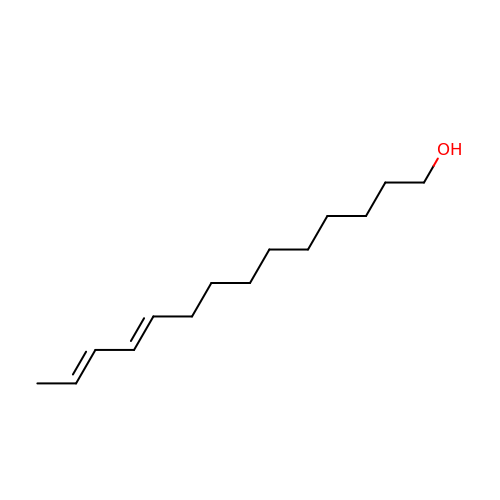(10E,12Z)-tetradeca-10,12-dien-1-ol | C14 H26 O | SDYZTPJTAFFSCK-AWYLAFAOSA-N>[2x]SFDPTGYTLAHEHLHIDLSGFKNNVDCRLDQYAFICQEMNDLMT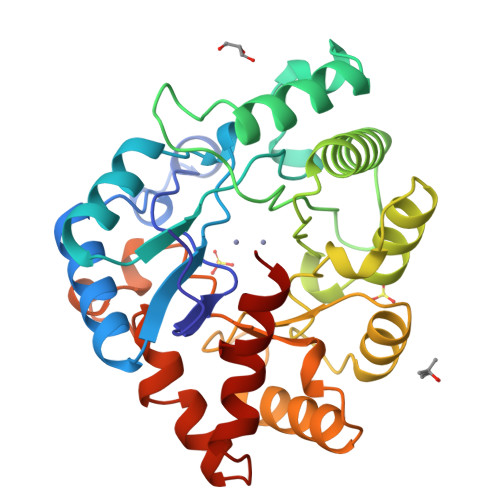RGVRNVIEMTNRYMGRNAQFMLDVMRETGINVVACTGYYQDAFFPEHVATRSVQELAQEMVDEIEQGIDGTELKAGIIAEIGTSEGKITPLEEKVFIAAALAHNQTGRPISTHTSFSTMGLEQLALLQAHGVDLSRVTVGHCDLKDNLDNILKMIDLGAYVQFDTIGKNSYYPDEKRIAMLHALRDRGLLNRVMLSMDITRRSHLKANGGYGYDYLLTTFIPQLRQSGFSQADVDVMLRENPSQFFQ>ARVGVLGAKGKVGATMVRAVAAADDLTLSAELDAGDPLSLLTDGNTEVVIDFTHPDVVMGNLEFLIDNGIHAVVGTTGFTAERFQQVESWLVAKPNTSVLIAPNFAIGAVLSMHFAKQAARFFDSAEVIELHHPHKADAPSGTAARTAKLIAEARKGLPPNPDATSTSLPGARGADVDGIP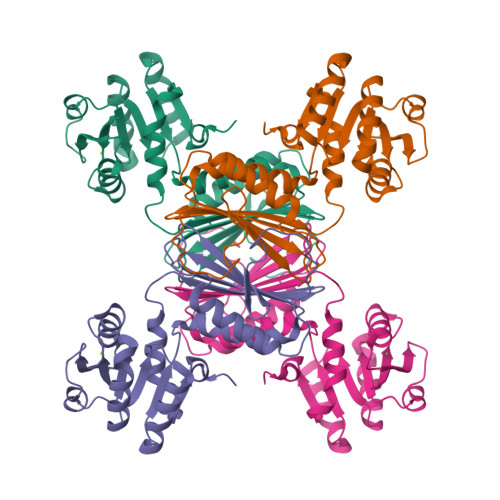VHAVRLAGLVAHQEVLFGTEGETLTIRHDSLDRTSFVPGVLLAVRRIAERPGLTVGLEPLLDLH[2x]~{N}-[3-[2-(dimethylamino)ethyl]-2-oxidanylidene-1,3-benzoxazol-5-yl]-1-methyl-6-oxidanylidene-pyridine-3-carboxamide 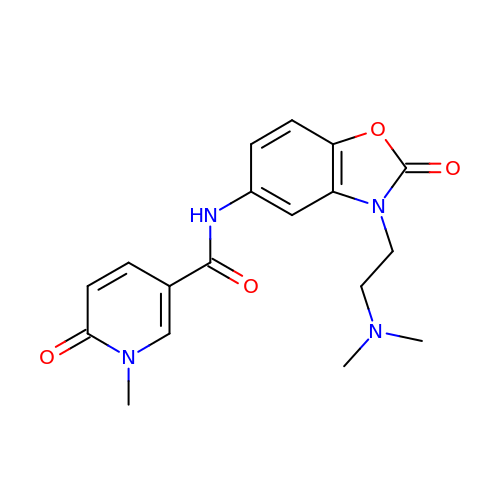| C18 H20 N4 O4 | RMQWPQCQFPMELT-UHFFFAOYSA-N> SSVVGLHYKIGKKIGEGSFGVIFEGTNIINGVPVAIKFEPRKTEAPQLRDEYRTYKHLQGCDGIPNAYYFGQE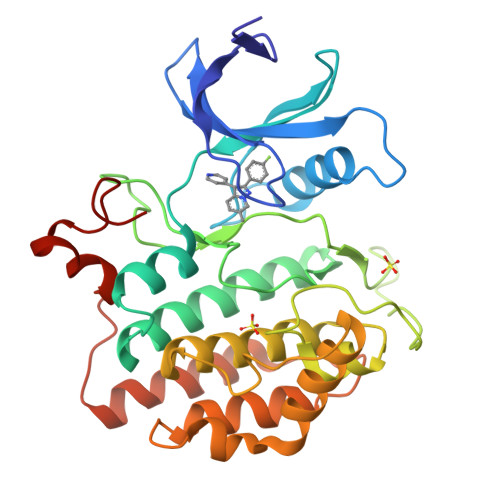GLHNILVIDLLGPSLEDLFDWCGRRFSVKTVVQVAIQMLTLVEEVHRHDLIYRDIKPDNFLIGRRGATDENNVHLIDFGMAKQYRDPRTKQHIPYREKKSLSGTARYMSINTHLGREQSRRDDLEALGHVFFYFLRGQLPWQGLKAPTNKQKYEKIGDKKRTTPAVTLCDGLPQQFAEYLDSVRSLPFDAEPPYEEYRMLLLSVLDDLGQACDGDMDWMHLNGGRGWDATINKKPN In this study, the effect of physical and chemical factors on the orientations of macromolecules was investigated through an analysis of selected well studied macromolecules, and important parameters that determine the behaviour of proteins on cryo-EM grids were revealed. The test proteins used in the analysis include human C-reactive protein (CRP) pentamer, CRP decamer, human erythrocyte catalase, SARS-CoV-2 spike protein, E. coli PaaZ and E. coli β-galactosidase. We performed a comprehensive examination of how macromolecule orientations respond to alterations in physical factors, such as freezing temperature, and chemical factors, such as the addition of surfactants or the presence of affinity tags, during grid freezing for a standard set of proteins. Hence, electrostatic interactions at the AWI are an important factor in determining protein orientations in the absence of any additive.

CRP exists in a concentration-dependent equilibrium between a pentamer and a decamer of a 25 kDa polypeptide under physiological conditions. In the concentration range used for cryo-EM experiments, both pentamer and decamer populations were observed in the same micrograph and were analysed separately. C5 symmetry was applied to the smaller pentameric molecule and no symmetry was applied to the decamer during image processing. The preferred view for the CRP pentamer is the top/bottom view, where the symmetric arrangement of the monomers can be seen. Some side views are observed, but no tilted side views are seen in the 2D class averages. The negatively charged B-face of CRP in the absence of additive is less sampled in the case of the CRP pentamer and is not sampled at all in the CRP decamer. However, we note that with CRP pentamer, the orientation distributions look similar with both Tween 20 and Tween 80, but only the addition of Tween 20 led to an isotropic map (R = 3.3 Å), while the addition of Tween 80 led to a low-resolution map (R = 7.5 Å). The orientations observed in this case look similar and the resulting reconstructions from 256 289 and 204 354 particles for the pentamer and decamer (C5 and C1 symmetry) resulted in resolutions of 3.2 and 2.8 Å, respectively. In comparison, we have obtained a 3.3 Å resolution map for the pentamer and a 4 Å resolution map for the decamer by averaging 25 000 and 51 000 particles, respectively.

>[5x]MEKLLCFLVLTSLSHAFGQTDMSRKAFVFPKESDTSYVSLKAPLTKPLKAFTVCLHFYTELSSTRGYSIFSYATKRQDNEILIFWSKDIGYSFTVGGSEILFEVPEVTVAPVHICTSWESASGIVEFWVDGKPRVRKSLKKGYTVGAEASIILGQEQDSFGGNFEGSQSLVGDIGNVNMWDFVLSPDEINTIYLGGPFSPNVLNWRALKYEVQGEVFTKPQLWP> MKNIFKIGLFALVTAFAMTSCDPQDGDDHSLGVKPQESQLSFTATPGSNPNVVTLKNT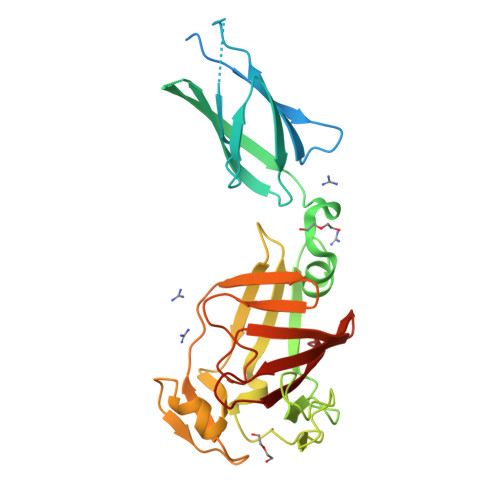SSLKGLVVTWDLGNGVTAKGEEVVASYPFANTYTIAMTAYNTGGSTTITQTITIANNDESQIEPKAIILAGGLTGSKTWVFDRAHDGHFGVGPGAGNPDYNGTPSWWSCPAEGKAECALYENEFSFHLDGGYNMTWVNKGKIYTNGAGKDKLPGVATVPGAGDFDVEYIPKEAYTFTVDGDKLKLSDDAFFGHFAGTSTYTIKTLNENELYLECSSAVESGNGWWYRFVPKK> MDRKVAREFRHKVDFLIENDAEKDYLYDVLRMYHQ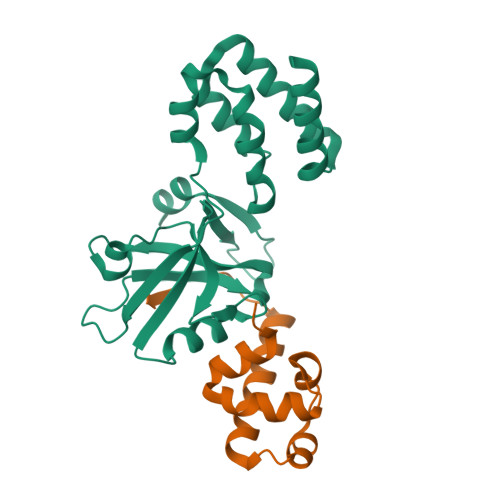TMDVAVLVGDLKLVINEPSRLPLFDAIRPLIPLKHQVEYDQLTPRRSRKLKEVRLDRLHPEGLGLSVRGGLEFGCGLFISHLIKGGQADSVGLQVGDEIVRINGYSISSCTHEEVINLIRTEKTVSIKVRHIGLIPVKSSPDEPLTWQYVDQFVSES;> ETSPLETFLASLHMEDFAALLRQEKIDLEALMLCSDLDLRSISVPLGPREKILGAVRRRRQAMERPPALEDTEL>[13x]MAEKRTGLAEDGAKSVYERLKNDRAPYETRAQNCAQYTIPSLFPKDSDNASTDYQTPWQAVGARGLNNLASKLMLALFPMQTWMRLTISEYEAKQLLSDPDGLAKVDEGLSMVERIIMNYIESNSYRVTLFEALKQLVVAGNVLLYLPEPEGSNYNPMKLYRLSSYVVQRDAFGNVLQMVTRDQIAFGALPEDIRKAVEGQGGEKKADETIDVYTHIYLDEDSGEYLRYEEVEGMEVQGSDGTYPKEACPYIPIRMVRLDGESYGRSYIEEYLGDLRSLENLQEAIVKMSMISSKVIGLVNPAGITQPRRLTKAQTGDFVTGRPEDISFLQLEKQADFTVAKAVSDAIEARLSFAFMLNSAVQRTGERVTAEEIRYVASELEDTLGGVYSILSQELQLPLVRVLLKQLQATQQIPELPKEAVEPTISTGLEAIGRGQDLDKLERCVTAWAALAPMRDDPDINLAMIKLRIANAIGIDTSGILLTEEQKQQKMAQQSMQMGMDNGAAALAQGMAAQATASPEAMAAAADSVGLQPGIAAALEHHHHHH

Phage portal proteins are key viral components located in a single pentameric vertex of the capsid and they act as initiators of capsid assembly. They are also critical components of the DNA-packaging complex and are involved in tail assembly. Here we report a number of crystal and high-resolution cryo-electron microscopy (cryo-EM) structures of the T7 bacteriophage portal (gp8). The structures show two conformations—open and closed—of the portal and suggest a possible mechanism of the channel valve that regulates DNA passage.

Several X-ray data sets from various crystal forms of the T7 portal in its dodecameric (12mer) and tridecameric (13mer) forms were collected. Although the portal protein is always found as a dodecamer in virions, assemblies containing 11–13 subunits have been described for other portals when expressed under non-physiological conditions. The T7 portal structure was finally solved by combining cryo-EM and X-ray crystallography. An initial map of the tridecameric form of the gp8 protein at 5.8 Å resolution was obtained by cryo-EM (gp8-13merEM). The ring-shaped volume allowed the ab-initio building of a partial poly-alanine model composed mainly of α-helices, which contained 36% of the structure. This partial model was later used for phasing a 3.4 Å resolution gp8-13mer crystallographic data set by molecular replacement and a full atomic model was built into the resulting electron density map (gp8-13mercryst). A deep cleft separates the wing and crown domains, which are connected only by a hinge at G434 between strand β13 of the wing and helix α11 of the crown. This feature confers some freedom of movement to the crown domain around that point, which is also supported by the fact that monomers from the dodecameric and tridecameric structures are very similar, except for the relative position of the crown domain respect to the rest of the protein (root mean squared deviation (RMSD) 0.849 Å).> GKDTSPKEMSVKPTAPQDKSVPVWNGFSLYTDDTVKAAAQYAYDNYLGKPYTGSVESAPANFGGRMVYRQHHGLSHTLRTMAYAELIVEEARKAKLRGETLGKFKDGRTIADVTPQELKKIMIAQAFFVAGRDDEASDAKNYQKYHEQSRDAFLKYVKDNESTLLPDVFKDQEDVNFYARVIEDKSHDWESTPAHVLINQGHMVDLVRVKQPPESFLQRYFSSMQRWIGSQATEAVFGIQRQFFHATYEVVAGFDSDNKEPHLVVSGLGRYVIGEDGQPIREAPKKGQKEGDLKVFPQTYKLKENERLMRVDEFLKLPEIQNTFPGSGKHLQGGMPGMNEMDYWNRLNSLNRARCENDVDFCLKQLQTAHDKAKIEPIKQAFQSSKGKERRQPNVDEIAAARIIQQILANPDCIHDDHVLINGQKLEQQFFRDLLAKCEMAVVGSLLNDTDIGNIDTLMRHEKDTEFHSTNPEAVPVKIGEYWINDQRINNSSGNITQKKHDLIFLMQNDAWYFSRVNAIAQNRDKGSTFKEVLITTLMTPLTSKALVDTSQAKPPTRLFRGLNLSEEFTKGLIDQANAMIANTTERLFTDHSPEAFKQIKLNDL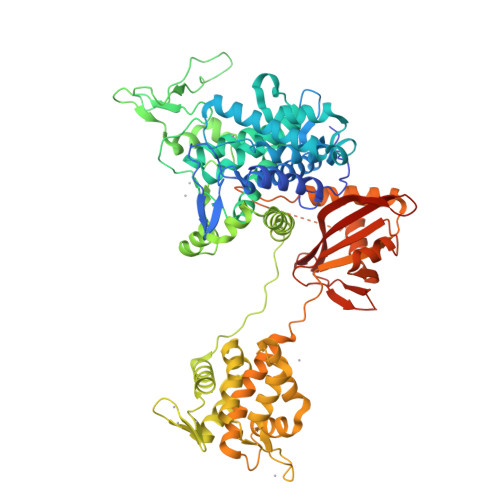SKMSGRTNASTTTEIKLVKETWDSNVIFEMLDPDGLLHSKQVGRHGEGTESEFSVYLPEDVALVPVKVTLDGKTQKGENRYVFTFVAVKSPDFTPRHESG>GSHMTSSANEDMPVERILEAELAVEPKTETYVEANMGLNPSSPNDPVTNICQAADKQLFTLVEWAKRIPHFSELPLDDQVILLRAGWNELLIASFSHRSIAVKDGILLATGLHVHRNSAHSAGVGAIFDRVLTELVSKMRDMQMDKTELGCLRAIVLFNPDSKGLSNPAEVEALREKVYASLEAYCKHKYPEQPGRFAKLLLRLPALRSIGLKCLEHLFFFKLIGDTPIDTFLMEMLEAPHQMT[2x];>[2x]KHKILHRLLQDSSSPVDLAKLTA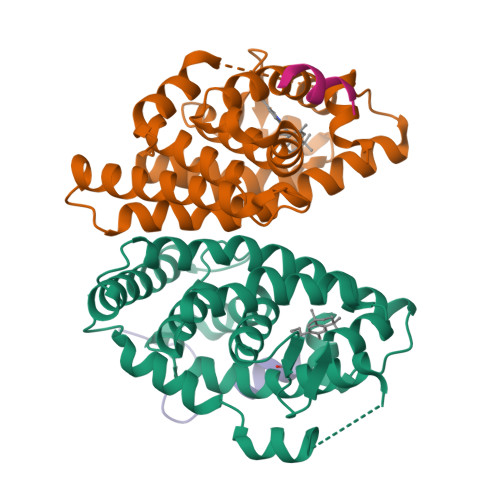EATGK> MARSNLLRDKKVEKEPI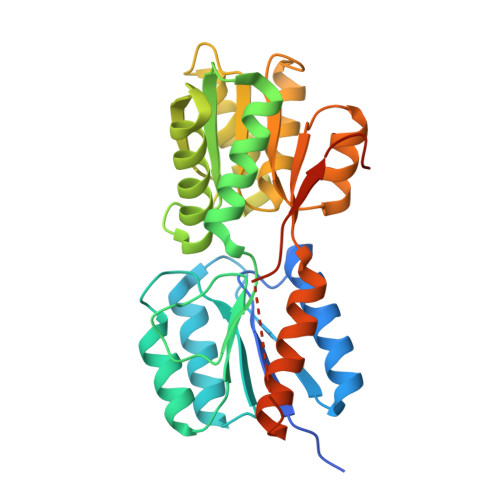KPKIVLISHIKTNPYWLDIKAGAERAAKERGAVVEFLGPTTASTEDGLKLFDMATSAKVSGIITYVQEEGQYKKKINSAMEKGIPVVTIDSDEEDSNRIAYVGTDNVLAGQVAGKEMVKQIGTSGNVAIVMGGKNVKNQKERVEGFTQYIKSNSNLKIVDTDSSDAMLLEAEIITRKILNRNDNINALFCTSALDGIGAARAVKDLNYKDRVKIICFDDLDDTLSNIRNGLVSATIVQKSNEMGYRAVNIIMDKIEGKSNKFSKSLIDVNVINKSDVDSYKRGDDKVEN> NPIHDRTSDYHKYLKVKQGDSDLFKLTVSDKRYIWYNPDPKERDSYECGEIVSETSDSFTFKTVDGQDRQVKKDDANQRNPIKFDGVEDMSELSYLNEPAVFHNLRVRYNQDLIYTYSGLFLVAVNPFKRIPIYTQEMVDIFKGRRRNEVAPHIFAISDVAYRSMLDDRQNQSLLITGESGAGKTENTKKVIQYLASVAGRNQANGSGVLEQQILQANPILEAFGNAKTTRNNNSSRFGKFIEIQFNSAGFISGASIQSYLLEKSRVVFQSETERNYHIFYQLLAGATAEEKKALHLAGPESFNYLNQSGCVDIKGVSDSEEFKITRQAMDIVGFSQEEQMSIFKIIAGILHLGNIKFEKGAGEGAVLKDKTALNAASTVFGVNPSVLEKALMEPRILAGRDLVAQHLNVEKSSSSRDALVKALYGRLFLWLVKKINNVLCQERKAYFIGVLDI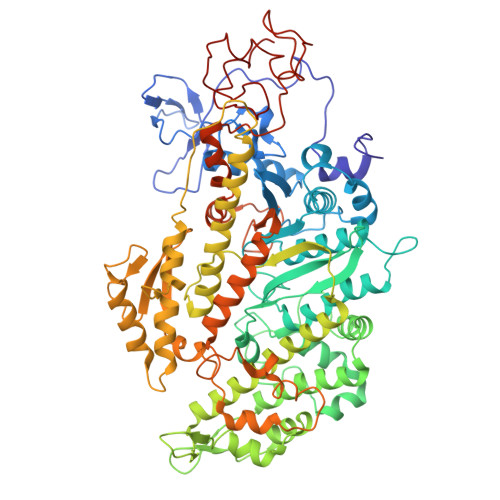SGFEIFKVNSFEQLCINYTNEKLQQFFNHHMFKLEQEEYLKEKINWTFIDFGLDSQATIDLIDGRQPPGILALLDEQSVFPNATDNTLITKLHSHFSKKNAKYEEPRFSKTEFGVTHYAGQVMYEIQDWLEKNKDPLQQDLELCFKDSSDNVVTKLFNDPNIASRAKKGANFITVAAQYKEQLASLMATLETTNPHFVRCIIPNNKQLPAKLEDKVVLDQLRCNAVLEGIRITRKGFPNRIIYADFVKRYYLLAPNVPRDAEDSQKATDAVLKHLNIDPEQYRFGITKIFFRAGQLARIEEARE>MRVKAAQAGRQSSAKRHLAEQFAVGEIITDMAAAAWKVGLPIGQGGFGCIYLADMNSSESVGSDAPCVVKVEPSDNGPLFTELKFYQRAAKPEQIQKWIRTRKLKYLGVPKYWGSGLHDKNGKSYRFMIMDRFGSDLQKIYEANAKRFSRKTVLQLSLRILDILEYIHEHEYVHGDIKASNLLLNYKNPDQVYLVDYGLAYRYCPEGVHKAYAADPKRC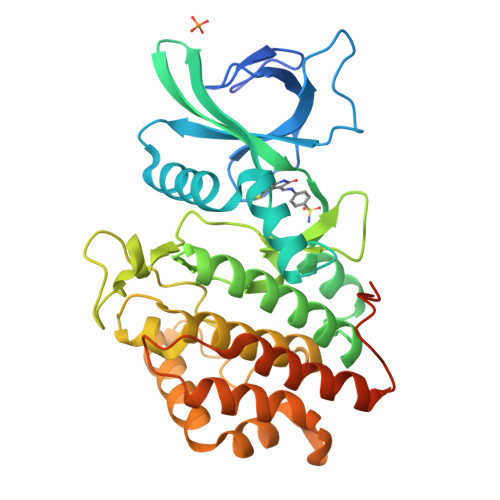HDGTIEFTSIDAHNGVAPSRRGDLEILGYCMIQWLTGHLPWEDNLKDPKYVRDSKIRYRENIASLMDKCFPAANAPGEIAKYMETVKLLDYTEKPLYENLRDILLQGLKAIGSKDDGKLDLSVVENGGLKAKTITKKRAAEIEE[4x]N-[2-(benzylamino)-2-oxoethyl]-4-(dimethylamino)-N-{[4-(hydroxycarbamoyl)phenyl]methyl}benzamide | C26 H28 N4 O4 | 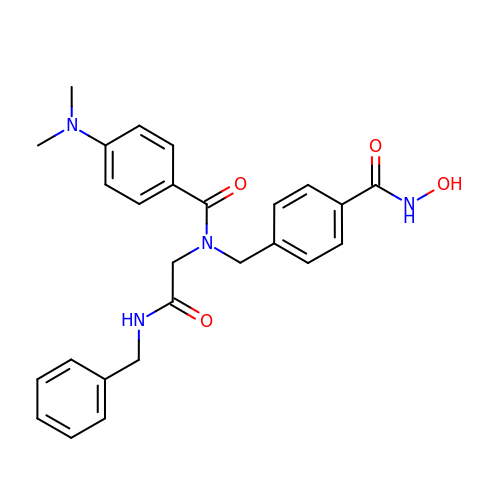WWCLIIDYSGNTQD-UHFFFAOYSA-N>[3x]MAGNRKLAVIGAGGHGKV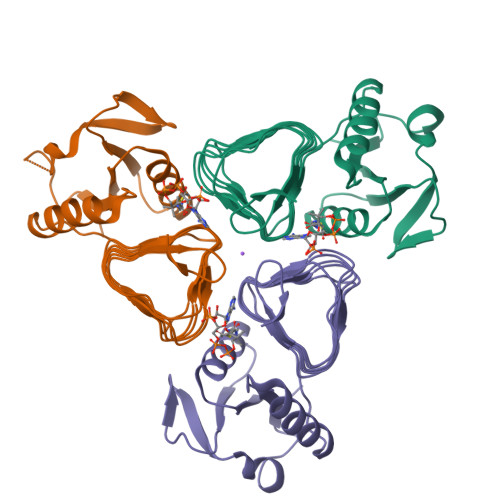VAELAAALGTYGEIVFLDDRTQGSVNGFPVIGTTLLLENSLSPEQFDITVAVGNNRIRRQITENAAALGFKLPVLIHPDATVSPSAIIGQGSVVMAKAVVQAGSVLKDGVIVNTAATVDHDCLLDAFVHISPGAHLSGNTRIGEESRIGTGACSRQQTTVGSGVTAGAGAVIVCDIPDGMTVAGNPAKPL> MADVPAGVTLAEKQTLVRNNGSEVQSLDPHKIEGVPESNISRDLFEGLLVSDLDGHPAPGVAESWDNKDAKVWTFHLRKDAKWSDGTPVTAQDFVYSWQRSVDPNTASPYASYLQYGHIAGIDEILEGKKPITDLGVKAIDDHTLEVTLSEPVPYFYKLLVHPSTSPVPKAAIEKFGEKWTQPGNIVTNGAYTLKDWVVNERIV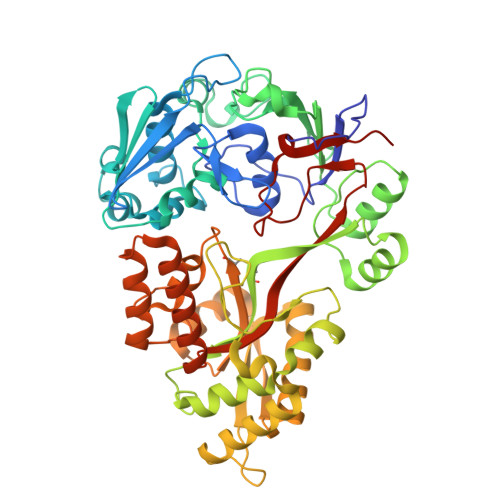LERSPTYWNNAKTVINQVTYLPIASEVTDVNRYRSGEIDMTNNSMPIELFQKLKKEIPDEVHVDPYLCTYYYEINNQKPPFNDVRVRTALKLGMDRDIIVNKVKAQGNMPAYGYTPPYTDGAKLTQPEWFGWSQEKRNEEAKKLLAEAGYTADKPLTINLLYNTSDLHKKLAIAASSLWKKNIGVNVKLVNQEWKTFLDTRHQGTFDVARAGWCADYNEPTSFLNTMLSNSSMNTAHYKSPAFDSIMAETLKVTDEAQRTALYTKAEQQLDKDSAIVPVYYYVNARLVKPWVGGYTGKDPLDNTYTRNMYIVKHHHHHHH> ETGNQDLPVIKCVLINHKNNDSSVGKSSSYPMVSESPEDLGCALRPQSSGTVYEAAAVEVDVSASITLQVLVDAPGNISCLWVFKHSSLNCQPHFDLQNRGVVSMVILKMTETQAGEYLLFIQSEATNYTILFTVSIRNTLLYTLRRPYFRKMENQDALVCISESVPEPIVEWVLCDSQGESCKEESPAVV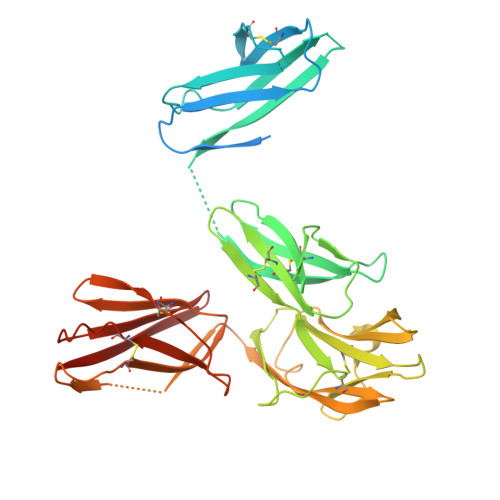KKEEKVLHELFGTDIRCCARNELGRECTRLFTIDLNQTPQTTLPQLFLKVGEPLWIRCKAVHVNHGFGLTWELENKALEEGNYFEMSTYSTNRTMIRILFAFVSSVARNDTGYYTCSSSKHPSQSALVTIVEKGFINATNSSEDYEIDQYEEFCFSVRFKAYPQIRCTWTFSRKSFPCEQKGLDNGYSISKFCNHKHQPGEYIFHAENDDAQFTKMFTLNIRSGTKHHHHHH5-(5-aminopent-1-yn-1-yl)-2'-deoxyuridine 5'-(tetrahydrogen 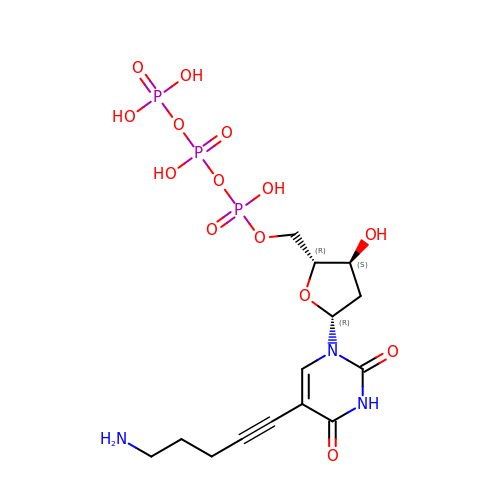triphosphate) | C14 H22 N3 O14 P3 | WENDCSLWIXFOST-QJPTWQEYSA-N> SHMFKVEIVTRPANFEKLKQELGKIGVTSLTFSNVHGCGLQKAHTELYRGVKIESNVYERLKIEIVVSKVPVDQVTETAKRVLKTGSPGDGKIFV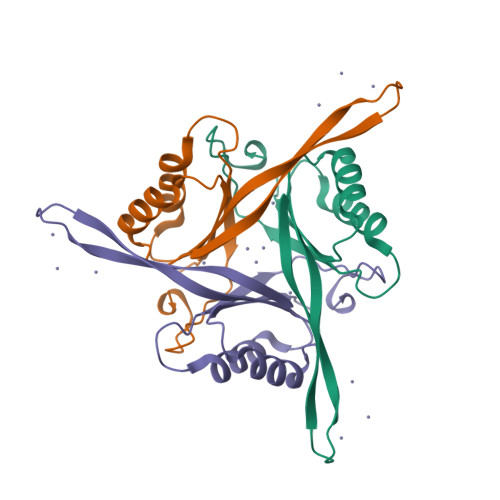YEISNTINIRTGEEGPEAL> GPHM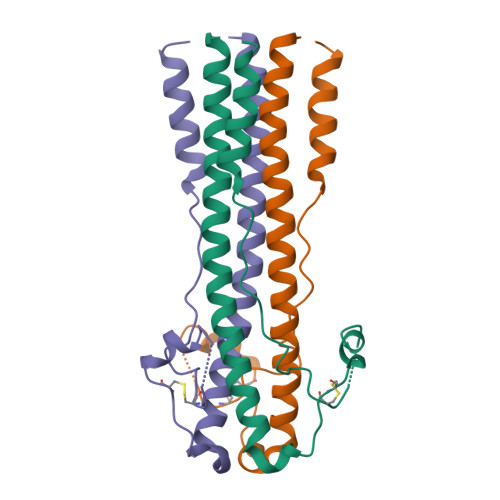DEEFSDMLRLFDFNKQAIQRLKAEAQMSIQLINKAVNALINDQLIMKNHLRDIMGIPYCNYSKYWYLNHTTTTSLPKCWLVSNGSYLNETHFSDDIEQQADNMITEMLQKEYMERQGKTPLGLVD>MIAHLINTDIGNRGVLKVYLDYRRKNFNFLHNSTKMFLDNLERVLIVTGFPIPPM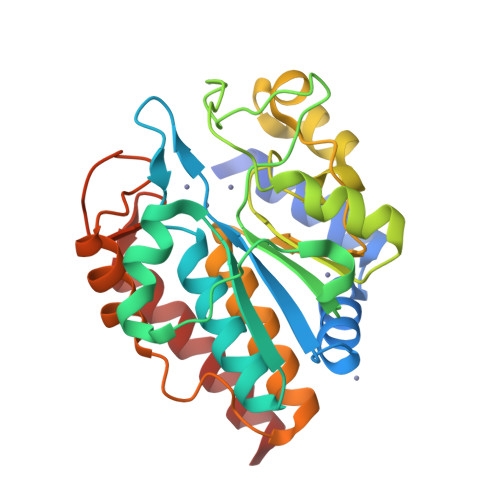MVAETDGPPGALAIYRAVEMLGGKAEILTYSEVEKALEPFGVSLARTPEPEDYSLIISVETPGRAADGRYYSMSALEIKRDPLDGIFLKARALGIPTIGVGDGGNEIGMGKIRELVVGHVPHGEKIASVVETDELIVSAVSNWGAYGLVAQASIEVGRNLLEGWDERRVIEAISSAGLIDGVSKTLAPSVDGIRLMVHEGIVELLKAVVDEAIL[6x]>[3x]GSHMFTGLNTPSGVAVDSAGTVYVTDHGNNRV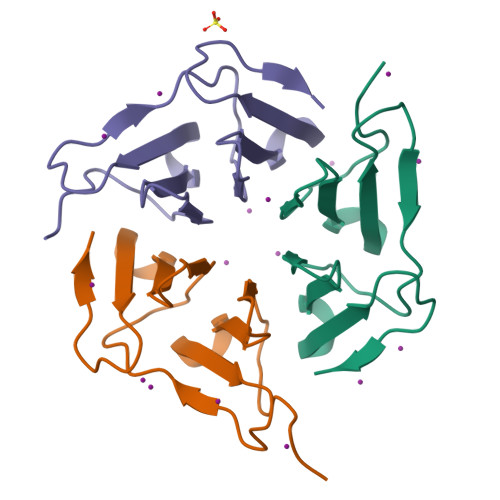VKLAAGSNTQTVLPFTGLNTPSGVAVDSAGTVYVTDHGNNRVVKLAAGSNTQTVL>[6x]MAEESRGQRGSGYGLGLSTRTQVTGYQFLARRTAMALTRWRVRMEIEPGRRQTLAVVASVSAALVICLGALLWSFISPSGQLNESPIIADRDSGALYVRVGDRLYPALNLASARLITGRPDNPHLVRSSQIATMPRGPLVGIPGAPSSFSPKSPPASSWLVCDTVATSSSIGSLQGVTVTVIDGTPDLTGHRQILSGSDAVVLRYGGDAWVIREGRRSRIEPTNRAVLLPLGLTPEQVSQARPMSRALFDALPVGPELLVPEVPNAGGPATFPGAPGPIGTVIVTPQISGPQQYSLVLGDGVQTLPPLVAQILQNAGSAGNTKPLTVEPSTLAKMPVVNRLDLSAYPDNPLEVVDIREHPSTCWWWERTAGENRARVRVVSGPTIPVAATEMNKVVSLVKADTSGRQADQVYFGPDHANFVAVTGNNPGAQTSESLWWVTDAGARFGVEDSKEARDALGLTLTPSLAPWVALRLLPQGPTLSRADALVEHDTLPMDMTPAELVVPK;>MKRGFARPTPEKPPVIKPENIVLSTPLSIPPPEGKPWWLIVVGVVVVGLLGGMVAMVFASGSHVFGGIGSIFPLFMMVGIMMMMFRGMGGGQQQMSRPKLDAMRAQFMLMLDMLRETAQESADSMDANYRWFHPAPNTLAAAVGSPRMWERKPDGKDLNFGVVRVGVGMTRPEVTWGEPQNMPTDIELEPVTGKALQEFGRYQSVVYNLPKMVSLLVEPWYALVGEREQVLGLMRAIICQLAFSHGPDHVQMIVVSSDLDQWD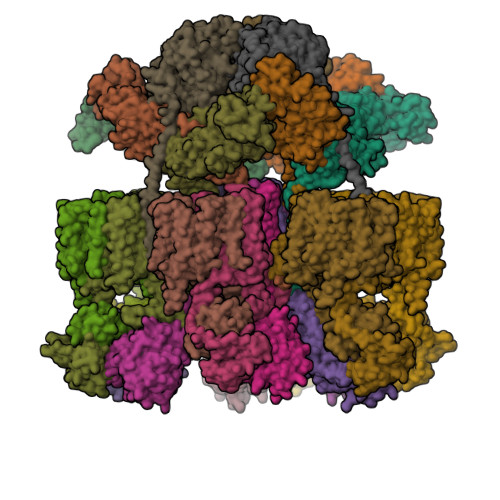WVKWLPHFGDSRRHDAAGNARMVYTSVREFAAEQAELFAGRGSFTPRHASSSAQTPTPHTVIIADVDDPQWEYVISAEGVDGVTFFDLTGSSMWTDIPERKLQFDKTGVIEALPRDRDTWMVIDDKAWFFALTDQVSIAEAEEFAQKLAQWRLAEAYEEIGQRVAHIGARDILSYYGIDDPGNIDFDSLWASRTDTMGRSRLRAPFGNRSDNGELLFLDMKSLDEGGDGPHGVMSGTTGSGKSTLVRTVIESLMLSHPPEELQFVLADLKGGSAVKPFAGVPHVSRIITDLEEDQALMERFLDALWGEIARRKAICDSAGVDDAKEYNSVRARMRARGQDMAPLPMLVVVIDEFYEWFRIMPTAVDVLDSIGRQGRAYWIHLMMASQTIESRAEKLMENMGYRLVLKARTAGAAQAAGVPNAVNLPAQAGLGYFRKSLEDIIRFQAEFLWRDYFQPGVSIDGEEAPALVHSIDYIRPQLFTNSFTPLEVSVGGPDIEPVVAQPNGEVLESDDIEGGEDEDEEGVRTPKVGTVIIDQLRKIKFEPYRLWQPPLTQPVAIDDLVNRFLGRPWHKEYGSACNLVFPIGIIDRPYKHDQPPWTVDTSGPGANVLILGAGGSGKTTALQTLICSAALTHTPQQVQFYCLAYSSTALTTVSRIPHVGEVAGPTDPYGVRRTVAELLALVRERKRSFLECGIASMEMFRRRKFGGEAGPVPDDGFGDVYLVIDNYRALAEENEVLIEQVNVIINQGPSFGVHVVVTADRESELRPPVRSGFGSRIELRLAAVEDAKLVRSRFAKDVPVKPGRGMVAVNYVRLDSDPQAGLHTLVARPALGSTPDNVFECDSVVAAVSRLTSAQAPPVRRLPARFGVEQVRELASRDTRQGVGAGGIAWAISELDLAPVYLNFAENSHLMVTGRRECGRTTTLATIMSEIGRLYAPGASSAPPPAPGRPSAQVWLVDPRRQLLTALGSDYVERFAYNLDGVVAMMGELAAALAGREPPPGLSAEELLSRSWWSGPEIFLIVDDIQQLPPGFDSPLHKAVPFVNRAADVGLHVIVTRTFGGWSSAGSDPMLRALHQANAPLLVMDADPDEGFIRGKMKGGPLPRGRGLLMAEDTGVFVQVAATEVRR[6x];>[12x]MTAVADAPQADIEGVASPQAVVVGVMAGEGVQIGVLLDANAPVSVMTDPLLKVVNSRLRELGEAPLEATGRGRWALCLVDGAPLRATQSLTEQDVYDGDRLWIRFIADTERRSQVIEHISTAVASDLSKRFARIDPIVAVQVGASMVATGVVLATGVLGWWRWHHNTWLTTIYTAVIGVLVLAVAMLLLMRAKTDADRRVADIMLMSAIMPVTVAAAAAPPGPVGSPQAVLGFGVLTVAAALALRFTGRRLGIYTTIVIIGALTMLAALARMVAATSAVTLLSSLLLICVVAYHAAPALSRRLAGIRLPVFPSATSRWVFEARPDLPTTVVVSGGSAPVLEGPSSVRDVLLQAERARSFLSGLLTGLGVMVVVCMTSLCDPHTGQRWLPLILAGFTSGFLLLRGRSYVDRWQSITLAGTAVIIAAAVCVRYALELSSPLAVSIVAAILVLLPAAGMAAAAHVPHTIYSPLFRKFVEWIEYLCLMPIFPLALWLMNVYAAIRYR;>[3x]MQRFGTGSSRSWCGRAGTATIAAVLLASGALTGLPPAYAISPPTIDPGALPPDGPPGPLAPMKQNAYCTEVGVLPGTDFQLQPKYMEMLNLNEAWQFGRGDGVKVAVIDTGVTPHPRLPRLIPGGDYVMAGGDGLSDCDAHGTLVASMIAAVPANGAVPLPSVPRRPVTIPTTETPPPPQTVTLSPVPPQTVTVIPAPPPEEGVPPGAPVPGPEPPPAPGPQPPAVDRGGGTVTVPSYSGGRKIAPIDNPRNPHPSAPSPALGPPPDAFSGIAPGVEIISIRQSSQAFGLKDPYTGDEDPQTAQKIDNVETMARAIVHAANMGASVINISDVMCMSARNVIDQRALGAAVHYAAVDKDAVIVAAAGDGSKKDCKQNPIFDPLQPDDPRAWNAVTTVVTPSWFHDYVLTVGAVDANGQPLSKMSIAGPWVSISAPGTDVVGLSPRDDGLINAIDGPDNSLLVPAGTSFSAAIVSGVAALVRAKFPELSAYQIINRLIHTARPPARGVDNQVGYGVVDPVAALTWDVPKGPAEPPKQLSAPLVVPQPPAPRDMVPIWVAAGGLAGALLIGGAVFGTATLMRRSRKQQ>[2x]MIYMLDTNIIIYLMKNRPKIIAERVSQLLPNDRLVMSF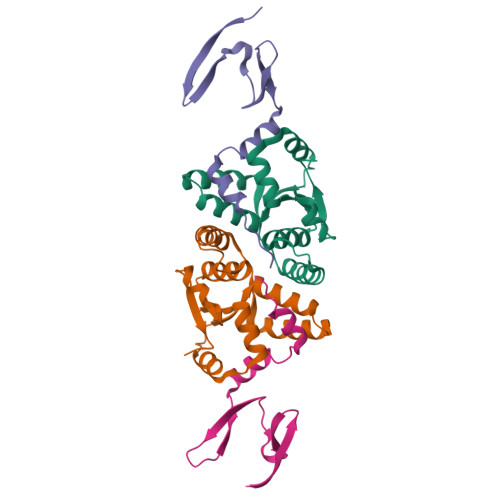ITYAELIKGAFGSQNYEQSIRAIELLTERVNVLYPNEQICLHYGKWANTLKKQGRPIGNNDLWIACHALSLNAVLITHNVKEFQRITDLQWQDWTKLLEHHHHHH;>MASMTGGQQMGRDPNSSSMLTKVFQSGNSQAVRIPMDFRFDVDTVEIFRKENGDVVLRPVSKKTDDFLALFEGFDETFIQALEARDDLPPQERENL[2x]>[2x]MSDKDSKNTPQVPEKLGLSRRGFLGASAVTGAAVAATALGGAVMTRESWAQAVKESKQKIHVGPGELDDYYGFWSGGHQGEVRVLGVPSMRELMRIPVFNVDSATGWGLTNESRHIMGDSAKFLNGDCHHPHISMTDGKYDGKYLFINDKANSRVARIRLDIMKCDKMITVPNVQAIHGLRLQKVPHTKYVFANAEFIIPHPNDGKVFDLQDENSYTMYNAIDAETMEMAFQVIVDGNLDNTDADYTGRFAAATCYNSEKAFDLGGMMRNERDWVVVFDIHAVEAAVKAGDFITLGDSKTPVLDGRKKD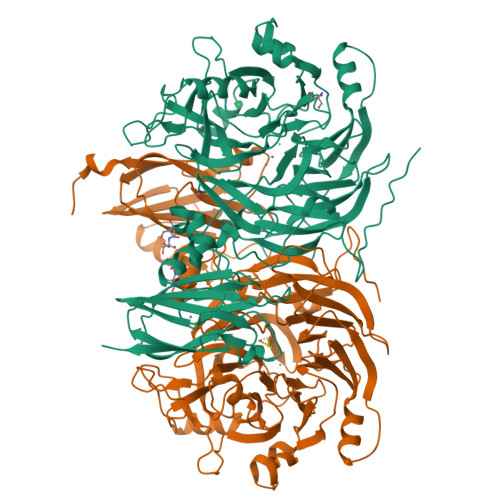GKDSKFTRYVPVPKNPHGCNTSSDGKYFIAAGKLSPTCSMIAIDKLPDLFAGKLADPRDVIVGEPELGLGPLHTTFDGRGNAYTTLFIDSQVVKWNMEEAVRAYKGEKVNYIKQKLDVHYQPGHLHASLCETNEADGKWLVALSKFSKDRFLPVGPLHPENDQLIDISGDEMKLVHDGPTFAEPHDCIMARRDQIKTKKIWDRNDPFFAPTVEMAKKDGINLDTDNKVIRDGNKVRVYMTSMAPAFGVQEFTVKQGDEVTVTITNIDQIEDVSEGFVVVNHGVSMEISPQQTSSITFVADKPGLHWYYCSWFCHALHMEMVGRMMVEPAWSHPQFEK>[2x]MNLKDKILGVAKELFIKNGYNATTTGEIVKLSESSKGNLYYHFKTKENLFLEILNIEESKWQEQWKSEQIKAKTNREKFYLYNELSLTTQYYYPLQNAIIEFYTEYYKTNSINEKMNKLENKYIDAYHVIFKEGNLNGEWSINDVNAVSKIAANAVNGIVTFTHEQNINERIKLMNKFSQIFLNGLSKHHHHHH

A member of the TetR family of transcriptional regulators, QacR is a dimer composed of nine alpha helices in which helices α1-3 comprise the helix-turn-helix (HTH) containing DNA-binding domain connected via helix α4 to helices α5-α9, which form the dimerization and multidrug-binding domain. QacR represses transcription of the qacA multidrug efflux transporter gene by binding as a pair of dimers to the IR1 DNA operator sequence, a large inverted repeat that overlaps the qacA promoter (PqacA). Drug binding occurs with a stoichiometry of one drug per QacR dimer and elicits a coil-to-helix transition of residues T89 through Y93 in the ligand-bound subunit resulting in the expulsion of Y92 and Y93 from the interior of the protein and the formation of the multidrug-binding pocket. The QacR multidrug-binding pocket contains two distinct but partially overlapping binding sites designated the rhodamine 6G (R6G) and ethidium (Et) sites after their respectively bound drugs.

Structures of QacR(E90Q) and QacR(E120Q) bound to Et, Dq, MG and R6G were solved to 2.8 Å, 3.3 Å, 2.2 Å and 2.9 Å resolution, or 3.3 Å, 2.9 Å, 2.4 Å and 3.2 Å resolution respectively. By contrast, QacR(E90Q) and QacR(E120Q) in complex with Et and MG crystallized in the hexagonal space group P62. Structural comparison of the hexagonal QacR mutant-drug complexes with the corresponding tetragonal wt QacR-drug complex revealed a new QacR conformation (with global RMSDs of ∼2.0 Å between all corresponding Cα atoms) in which notably, residues 89 through 93 had undergone the coil-to-helix transition, the structural hallmark of drug-mediated induction. Thus, the hexagonal form of QacR exhibits a closer approach of the DNA-binding domains, and therefore the recognition helices, with their centre-to-centre distance now 39.1 Å compared with 46.4 Å for the tetragonal conformer. Although charge neutralization of Et was ascribed solely to E120 in the wt QacR-drug complex, the location of Et in the QacR(E90Q)-Et structure is dramatically altered. In this QacR(E90Q)-Et complex, Et is angled at 120° relative to its wt orientation and shifted toward the R6G sub-pocket, hence overlapping the Et and R6G sub-pockets and taking a position that is comparable to that occupied by MG. Lost are van der Waals contacts with the side chains of I99 and I100 and aromatic stacking interactions with F162′ and Y103, the latter residue shifting from a position that would have clashed with Et in the QacR(E90Q)-Et structure. Nevertheless, Et gains stacking interactions with W61 and van der Waals contacts with S86, M116 and N154. Indeed, in the QacR(E90Q)-Et structure, the side chain of E120, despite remaining within 4 Å of the Et phenanthridinium ring system, is repositioned to avoid a clash with the drug, shifting by 3.0 Å so that it is no longer available to charge complement the Et N5 nitrogen atom (E120-N5 distance  = 4.0 Å in the wt QacR-Et complex and 7.0 Å in the QacR(E90Q)-Et complex).>GSHMVTIVRIYLDGVYGIGKSTTGRVMASAASGGSPTLYFPEPMAYWRTLFETDVISGIYDTQNRKQQGNLAVDDAALITAHYQSRFTTPYLILHDHTCTLFGGNSLQRGTQPDLTLVFDRHPVASTVCFPAARYLLGDMSMCALMAMVATLPREPQGGNIVVTTLNVEEHIRRLRTRAR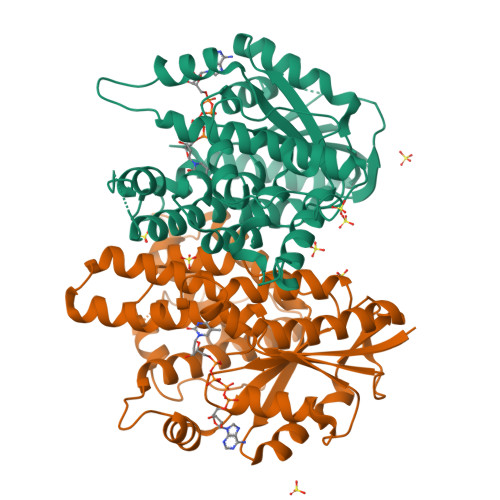IGEQIDITLIATLRNVYFMLVNTCHFLRSGRVWRDGWGELPTSCGAYKHRATQMDAFQERVSPELGDTLFALFKTQELLDDRGVILEVHAWALDALMLKLRNLNVFSADLSGTPRQCAAVVESLLPLMSSTLSDFDSASALERAARTFNAEMGV[4x]> ARQIVLASRPVGAPTAENFALTQSDIPTPAQGEMLLRSVYLSLDPYMRGRMSDAKSYAEPVGIDEVMVGGTVCQVEASNHAEFEVGEWVLAYTGWQDYAISDGEGLIKLGKQPSHPSYALGVMGMPGFTAYMGLLDIGQPKEGDTLVVAAATGAVGSMVGQIGKLKGCRVIGIAGGEEKCQFAKDTLGFDECID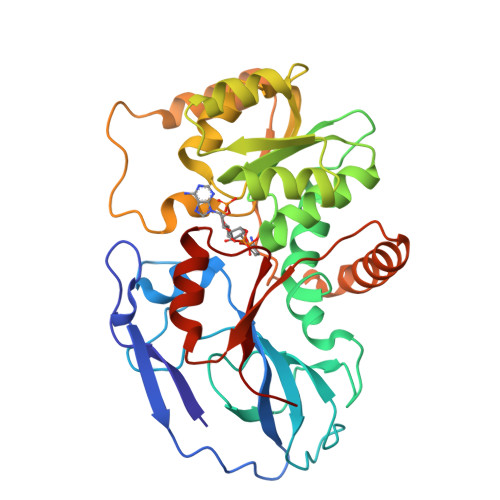HKAADFAEQLAKVCHNGIDIYFENVGGKVFDAVMPLLNTGARIPLCGLISQYNATSLPEGPDRMSMLMAQLLIKRIKMQGFIIFDDYGHRYGEFAADMTQWLAQGKIHYREHLVQGLENAPDAFIGLLEGKNFGKMVVQTNQP However, a freestanding enzyme D-aminoacyl-tRNA deacylase (DTD) removes D-amino acids (D-aas) mischarged on tRNAs and ensures that D-aas do not get incorporated into proteins. Mechanistically, the most remarkable challenge that DTD faces is to specifically act on multiple D-aa-tRNAs while rejecting L-aminoacyl-tRNAs (L-aa-tRNAs) without any specificity for either the amino acid or the tRNA. The enzyme is a symmetric dimer with two active sites per dimer that are located at the dimeric interface. A mechanistically unique solution to the problem of enantioselectivity employing two carbonyl oxygens from a ‘cross-subunit’ Gly-cisPro dipeptide has been shown to be responsible for D-chirality selection and strict L-chirality rejection from the active site of DTD.

PfDTD was co-crystallized with a post-transfer substrate analog D-Tyr3AA, which mimics D-tyrosine attached to the 3′-OH of the terminal adenosine (A76) of tRNA. Similar post-transfer substrate analogs have been used extensively to study proofreading mechanisms in atomic details for both Class I-specific CP1 editing domains and Class II-specific editing domains.The crystal structure of PfDTD in complex with D-Tyr3AA has been solved in two different crystal forms: crystal form I at a resolution of 1.86 Å in C2 space group and crystal form II at a resolution of 2.2 Å in P21 space group. Crystal forms I and II have two and eight copies per asymmetric unit, respectively. Since all copies present a similar picture, the higher resolution crystal form I is discussed here unless otherwise mentioned. An invariant Phe137 provides base-stacking interaction to the adenine ring. The main chain nitrogen of Gly138 along with the side chain hydroxyl of Ser87 holds the 2′-OH. The α-amino group of D-tyrosine has an interaction with carbonyl oxygen of Gly149 from the cross-subunit Gly-cisPro motif. Such a capture of the carbonyl oxygen and the amino group of the incoming D-aa, automatically positions the Cβ in such a way that it makes favorable C-H…O hydrogen bond with the carbonyl oxygen of Pro150, again from the cross-subunit Gly-cisPro motif. The cis conformation of Pro150 is the key to ensuring that it cradles the chiral centre thus preventing both the amino group and the Cβ from occupying the position of Hα.

>[2x]MRVVIQRVKGAILSVRKENIGENEKELEIISEIKNGLICFLGIHKNDTWEDALYIIRKCLNLRLWNNDNKTWDKNVKDLNYELLIVSQFTLFGNTKKGNKPDFHLAKEPNEALIFYNKIIDEFKKQYNDDKIKIGKFGNYMNIDVTNDGPVTIYIDTHDINLNK>[2x]PHEELQYLRQLREILCRGSDRLDRTGIGTLSLFGMQARYSLRDHFPLLTTKRVFWRGVVQELLWFLKGSTDSRELSRTGVKIWDKNGSREFLAGRGLAHRREGDLGPVYGFQWRHFGAAYVDADADYTGQGFDQLSYIVDLIKNNPHDRRIIMCAWNPADLSLMALPPCHLLCQFYVADGELSCQLYQRSGDMGLGVPFNIASYSLLTYMLAHVTGLRPGEFIHTLGDAHIYKTHIEPLRLQLTRTPRPFPRLEILRSVSSMEEFTPDDFRLVDYCPHPTIRMEM

TS is an essential enzyme for DNA replication. It catalyzes the transfer of a methylene group from the cofactor 5,10-methylenetetrahydrofolate (mTHF) to its substrate 2′-deoxyuridine-5′-monophosphate (dUMP) and produces thymidine-5′-monophosphate (dTMP) and dihydrofolate (DHF). KSHV encodes functional thymidylate synthase (kTS), which shares 70% sequence identity with hTS. The overall structure of kTS was found to have a similar structural conformation to hTS, except minor differences in ligand binding site and conformational variations in some amino acids.

Although co-crystallization of kTS protein with ligands was unsuccessful, binary and ternary kTS structures were obtained by soaking apo kTS crystals with dUMP and/or raltitrexed. Three Arg residues (Arg199’, Arg200’, and Arg239) of binary and ternary kTS structures had direct contacts with the phosphate group of dUMP, which were consistently observed in other TS structures. The loop region (residues 71–79) of apo and ternary kTS structures was shifted away from the phosphate group, and the subsequent Arg74 residue was tilted out; on the other hand, the Arg74 residue of binary kTS was coordinated around the phosphate group of dUMP as observed in other TS structures. However, the loop region (Arg71–Thr79) containing Arg74 in the binary complex of kTS had a similar orientation to other TS structures. In binary complex of kTS, this C-terminal region was well occupied around the ligand binding site, but it did not contribute to a closed conformation. The C-terminal region was observed in the binary kTS structure, but with an open conformation. As calculated above, the distance across active site was over 18.5 Å in other TS structures with an open conformation, including rTS, binary kTS, and vTS structures; however, a shorter distance of 17.9 Å in ecTS demonstrated a closed conformation.> MGEETYEGTSGREGGRHEEEVETRAARESAEEVWGGTEDLTSLSVEELKGLLARFDEEEKRISYRRRVIQGRIDVIRAEIVRRGGAVLSPEELARVLMGDVGDES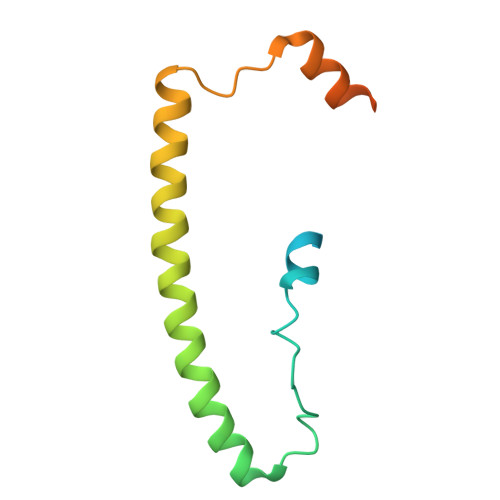EGGASGDRRGDGA>MGSHHHHHHSAALEVLFQGPGGNGKLRQWLIDQIDSGKYPGLVWENEEKSIFRIPWKHAGKQDYNRE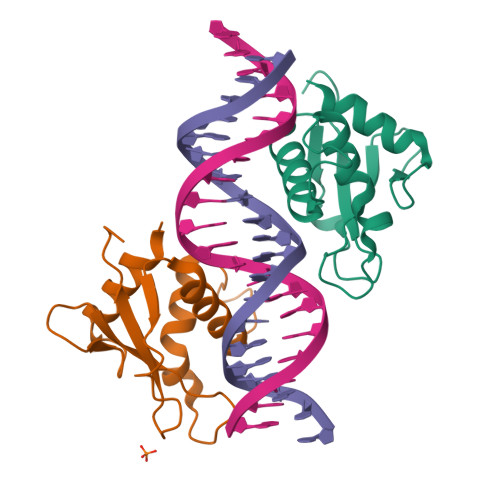EDAALFKAWALFKGKFREGIDKPDPPTWKTRLRCALNKSNDFEELVERSQLDISDPYKVYRIVPEGAKKGAKQL[2x]> MAATAAEAVASGSGEPREEAGALGPAWDESQLRSYSFPTRPIPRLSQSDPRAEELIENEEPVVLTDTNLVYPALKWDLEYLQENIGNGDFSVYSASTHKFLYYDEKKMANFQNFKPRSNREEMKFHEFVEKLQDIQQRGGEERLYLQQTLNDTVGRKIVMDFLGFNWNWINKQQGKRGWGQLTSNLLLIGMEGNVTPAHYAEQQNFFAQIKGYKRCILFPPDQFECLYPYPVHHPCDRQSQVDFDNPDYERFPNFQNVVGYETVVGPGDVLYIPMYWWHHIESLLNGGITITVNFWYKGAPTPKRIEYPLKAHQKVAIMRNIEKMLGEALGNP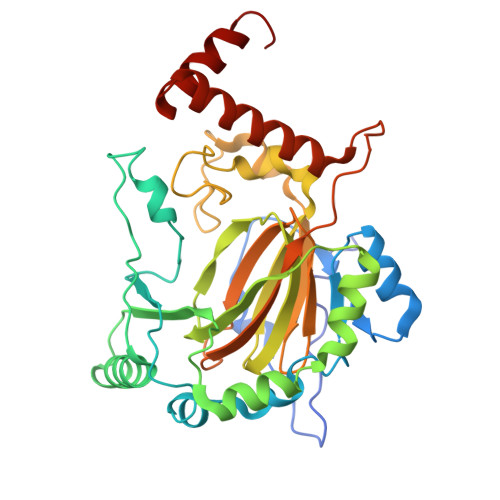QEVGPLLNTMIKGRYN>GPKTLKFMTASSPLSPKDPNEKLILQRLEKETGVHIDWTNYQSDFAEKRNLDISSGDLPDAIHNDGASDVDLMNWAKKGVIIPVEDLIDKYMPNLKKILDEKPEYKALMTAPDGHIYSFPWIEELGDGKESIHSVNDMAWINKDWLKKLGLEMPKTTDDLIKVLEAFKNGDPNGNGEADEIPFSFISGNGNEDFKFLFAAFGIGDNDDHLVVGNDGKVDFTADNDNYKEGVKFIRQLQEKGLIDKEAFEHDWNSYIAKGHDQKFGVYFTWDKNNVTGSNESYDVLPVLAGPSGQKHVARTNGMGFARDKMVITSVNKNLELTAKWIDAQYAPLQSVQNNWGTYGDDKQQNIFELDQASNSLKHLPLNGTAPAELRQKTEVGGPLAILDSYYGKVTTMPDDAKWRLDLIKEYYVPYMSNVNNYPRVFMTQEDLDKIAHIEADMNDYIYRKRAEWIVNGNIDTEWDDYK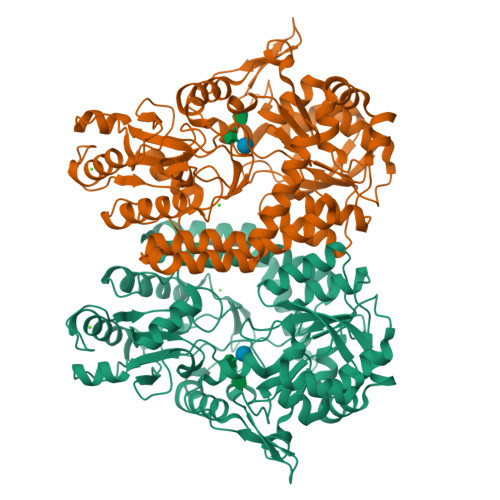KELEKYGLSDYLAIKQKYYDQYQANK[4x]> MGSLPCDICKDVVTAAGDMLKDNATEEEILVYL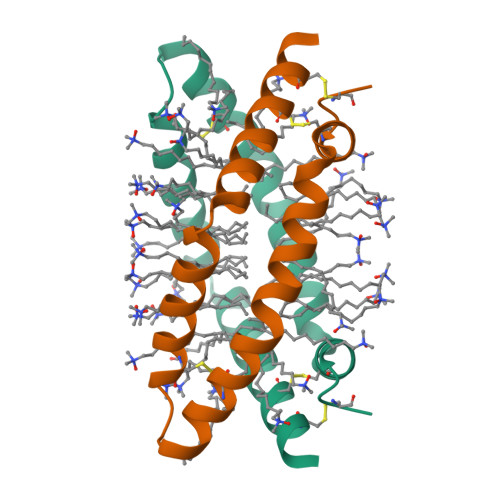EKTCDWLPKPNMSASCKEIVDSYLPVILDIIKGEMSRPGEVCSALNLCES> MKLRRKS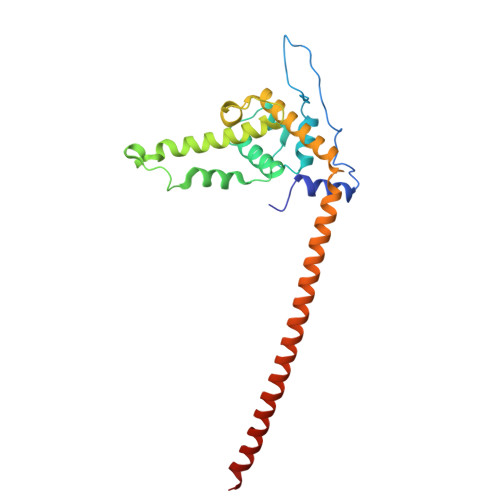ILHTIRNSIASGARISLGSGAARVVNGPVSRNQDVFPILDLQELVICLQSCDFALATQENISRPTSDYMVTLYKQIIENFMGISVESLLNSSNQETGDGHLQEENENIYLDTLNVLVLNKICFKFFENIGVQDFNMTDLYKPEAQRTQRLLSAVVNYARFREERMFDCNSFILQMESLLGQINKLNDEIKQLQKDFEVEVKEIEIEYSLLSGHINKYMNEMLEYMQ> MWELTILHTNDVHSRLEQTSEDSSKCVDASRCMGGVARLFTKVQQIRRAEPNVLLLDAGDQYQGTIWFTVYKGAEVAHFMNALRYDAMALGNHEFDNGVEGLIEPLLKEAKFPILSANIKAKGPLASQISGLYLPYKVLPVGDEVVGIVGYTSKETPFLSNPGTNLVFEDEITALQPEVDKLKTLNVNKIIALGHSGFEMDKLIAQKVRGVDVVVGGHSNTFLYTGNPPSKEVPAGKYPFIVTSDDGRKVPVVQAYAFGKYLGYLKIEFDERGNVISSHGNPILLDSSIPEDPSIKADINKWRIKLDDYSTQELGKTIVYLDGSSQSCRFRECNMGNLICDAMINNNLRHADEMFWNHVSMCILNGGGIRSPIDERNDGTITWENLAAVLPFGGTFDLVQ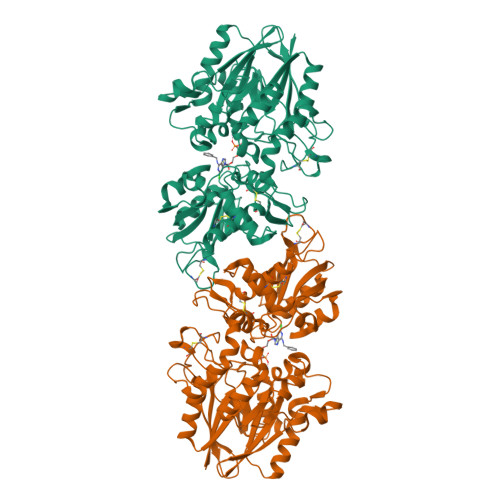LKGSTLKKAFEHSVHRYGQSTGEFLQVGGIHVVYDLSRKPGDRVVKLDVLCTKCRVPSYDPLKMDEVYKVILPNFLANGGDGFQMIKDELLRHDSGDQDINVVSTYISKMKVIYPAVEGRIKFSLEHHHHHH>KRKFACVECRQQKSKCDAHERAPEPCTKCAKKNVPCILKRDFRRTYKRARNEAIEKRFKELTRTLT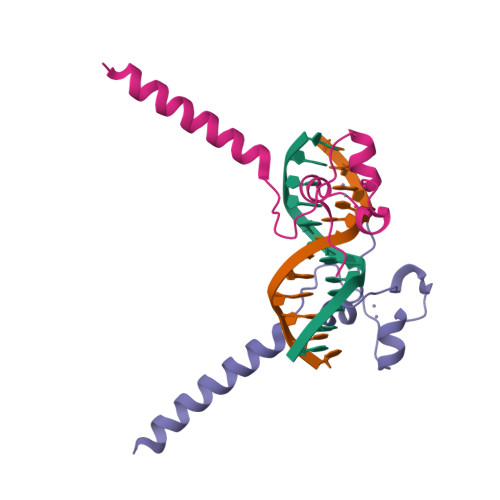NLTSDE[4x]>GPLGSPEFNNIENIGDGAEVVKRTEDTSSDKWGVTQNIQFDFVKDKKYNKDALILKMQGFINSKTTYYNYKNTDHIKAMRWPFQYNIGLKTNDPNVDLINYLPKNKIDSVNVSQTLGYNIGGNFNSGPSTGGNGSFNYSKTISYNQQNYISEVEHQNSKSVQWGIKANSFITSLGKMSGHDPNLFVGYKPYSQNPRDYFVPDNELPPLVHSGFNPSFIATVSHEKGSGDTSEFEITYGRNMDVTHATRRTTHAGNSYLEGSRIHNAFVNRNYTVKYEVNWKTHEIKVKGHN[4x]

With the exception of α-hemolysin, which is homo-heptameric, leukotoxins are bipartite toxins, formed by the non-covalent association of two distinct proteins, a class S and a class F component of approximately 31 and 34 kDa, respectively, into a likely octameric species. Panton-Valentine leukocidin (PVL) is associated with necrotizing skin infections, such as boils, and plays an important role in the poor prognosis of necrotizing pneumonia. Two additional structural domains are also found: the rim domain anchors the protein to the membrane surface, while the stem domain, closely apposed to the core β-sandwich in the soluble form, contributes two β-strands to the pore β-barrel. Since the binding of LukS-PV to the membrane is a saturable process, the necessary presence of a LukS-PV receptor on the cell surface was thus proposed. This was recently confirmed by Spaan et al. who showed that the C5a receptor is required for the binding of LukS-PV to human neutrophils.

Five mutants (Y181A, K182A, H245A, Y246A and N248A) were partially affected. LukS-PV mutants Y181A, K182A, Y246A and N248A also had a significantly decreased calcium entry slope, from 65% to 75% of the control (p<0.05, one-way ANOVA). The T244A, Y246A and N248A mutated proteins crystallized in identical conditions (50% PEG 200, 0.1 M MES-NaOH, pH 7.50). The corresponding crystals belonged to the P43212 space group, with similar cell parameters (a = b∼94 Å and c∼308 Å) and 4 molecules per asymmetric unit. These crystals diffracted X-rays at medium resolution (2.50 to 2.80 Å). In the case of the rim domain, wild-type LukS-PV and mutants T244A, Y246A and N248A displayed only small differences, with r.m.s. deviations comprised between 0.20 Å and 0.30 Å, whereas the structure of the rim domain of the Y184A and Y250A mutants were markedly different, with r.m.s. deviations of 1.10 Å and 1.28 Å, respectively, when compared to the wild-type LukS-PV structure. In close proximity to residues Y184, T244 and Y250, residues R242, H245 and Y246 also induced altered biological activities when mutated to alanine, albeit to a somewhat lesser extent. Residues R73, H245, Y246 and N248 are specific to the two proteins, whereas Y184 of LukS-PV is replaced by a histidine residue in HlgC.>[3x]MANVDEAILKRVKGWAPYVDAKLGFRNHWYPVMFSKEINEGEPKTLKLLGENLLVNRIDGKLYCLKDRCLHRGVQLSVKVECKTKSTITCWYHAWTYR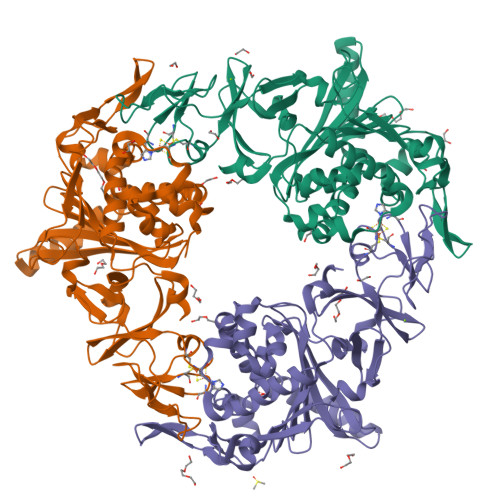WEDGVLCDILTNPTSAQIGRQKLKTYPVQEAKGCVFIYLGDGDPPPLARDTPPNFLDDDMEILGKNQIIKSNWRLAVENGFDPSHIYIHKDSILVKDNDLALPLGFAPGGDRKQQTRVVDDDVVGRKGVYDLIGEHGVPVFEGTIGGEVVREGAYGEKIVANDISIWLPGVLKVNPFPNPDMMQFEWYVPIDENTHYYFQTLGKPCANDEERKKYEQEFESKWKPMALEGFNNDDIWAREAMVDFYADDKGWVNEILFESDEAIVAWRKLASEHNQGIQTQAHVSGLEHHHHHH> TAHRFLFVSTPVGPLGSGRGGGVELTLPNLAKALTQRGHQVSVLAPAGSVLPDLPLETVPGTWQSTAQSHGRATPAEIPAESVLARLWDRAHQQQADFDLILNFAYDWLPLYLTPFFKTPVAHLISMGSLSEVMDQAIATSLDRYPGSIAVHSLAQAATFPFGDRCLCIGNALDLAAYGFNPEPEPVLGWVGRIAPEKGLEDAIQAAQQAGLPLRVWGALTEPDYWQRLQQQFGDRAVSYQGFVSTDELQRGLGRCQGLLMTPKWVEAFGNVAIEALACGLPVIAYARGGPLEIIEQGKSGWLVEPDQQAALVNAIGQLSSLDRAYCRAQAEARFSLAAMGQRLEAWLLPLLSR;> TAHRFLFVSTPVGPLGSGRGGGVELTLPNLAKALTQRGHQVSVLAPAGSVLPDLPLETVPGTWQSTAQSHGRATPAEIPAESVLARLWDRAHQQQADFDLILNFAYDWLPLYLTPFFKTPVAHL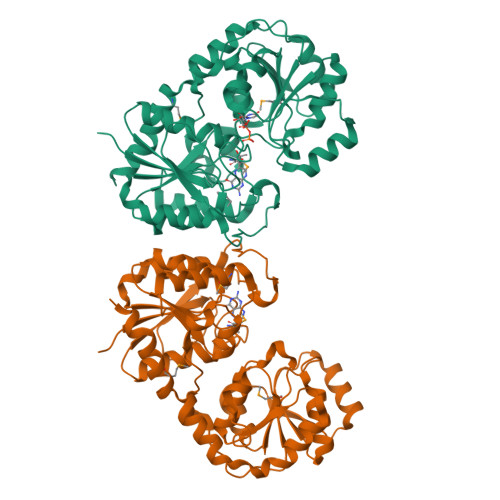ISMGSLSEVMDQAIATSLDRYPGSIAVHSLAQAATFPFGDRCLCIGNALDLAAYGFNPEPEPVLGWVGRIAPEKGLEDAIQAAQQAGLPLRVWGALTEPDYWQRLQQQFGDRAVSYQGFVSTDELQRGLGRCQGLLMTPKWVEAFGNVAIEALACGLPVIAYARGGPLEIIEQGKSGWLVEPDQQAALVNAIGQLSSLDRAYCRAQAEARFSLAAMGQRLEAWLLPLLS N-{(1S,2R)-1-benzyl-2-hydroxy-3-[(3-methoxybenzyl)amino]propyl}-5-[methyl(methylsulfonyl)amino]-N'-[(1R)-1-phenylethyl]benzene-1,3-dicarboxamide 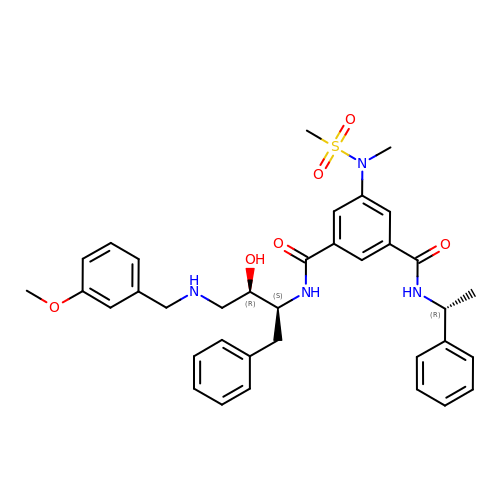| C36 H42 N4 O6 S | HIQWWDCRULXYDF-SWROZOJRSA-N>[20x]MLFFVDTANIDEIREANELGILAGVTTNPSLVAKEANVSFHDRLREITDVVKGSVS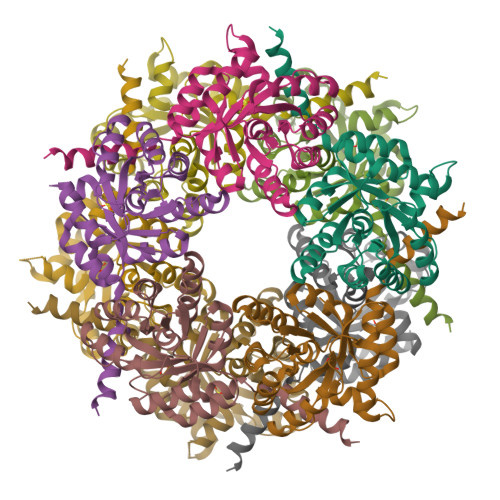AEVISLKAEEMIEEGKELAKIAPNITVKIPMTSDGLKAVRALTDLGIKTNVTLIFNANQALLAARAGATYVSPFLGRLDDIGHNGLDLISEVKQIFDIHGLDTQIIAASIRHPQHVTEAALRGAHIGTMPLKVIHALTKHPLTDKGIEQFLADWNK C2-1-HYDROXY-3-METHYL-PROPYL-THIAMIN 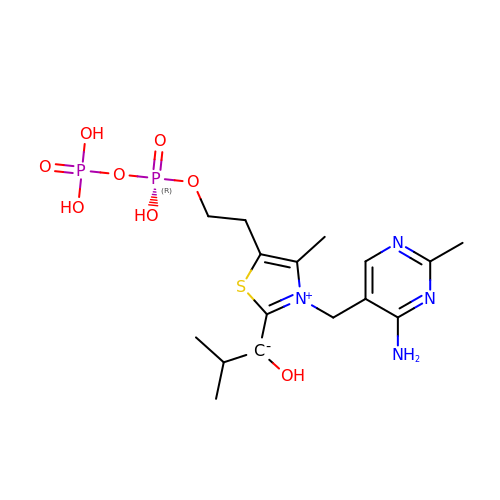DIPHOSPHATE | C16 H26 N4 O8 P2 S | VBABUKBBNKNHAI-UHFFFAOYSA-N>[2x]QNVGTQAAEEPLNLPISVCTAPGNCQTEADAVVLDSNWRWAHTTTGYTNCYTGNLWDTTLCPT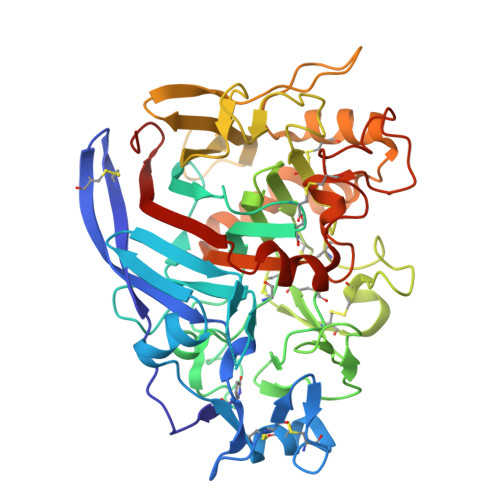PETCTTNCAIDGVPLADWSGTYGGSVTGNKFNLKFVTVGPYSTNIGARTFLLDSTKTRYRMFQLLNREFTYDVDVSSLDCGLNGALYFVSMDADGGAAKYPTNKGGAKYGTGYCDAQCPHDVKWINGLANSKDWTPIPGDANSGKGYYGNCCAELDIWEANKQSQAFTTHPCTPNDQTRCEGVVCGDNDSGDRYNGMCDKDGCDFASYRMNDHTFYGPGSTFKLDSTKPFTVVSQFITTDGTDNGDFKEFRRFYVQNGVRIENSKVNFPGITAYDSITDEMCAATKGLFGDLDDHKNKGGMKQMGEAMRKGMALVMSIWDDHDVNMLWLDSNYPPTGNPSTPGVARGPCPTTSGVPSEVEVTQANAVVSFGNIKFGPIGSTV>MSTLKNTFFITPPDTPTQAGPENIFYDFNDGARVLLPEGKWHVRLLDADSENILFCCDVDKGWVTSSKKYFVRFRIQVFRQGAATPLLDETLKLKDRPVLISFPTGTLGDLLGWFPYAERFQSLHKCRLECTMSQDIIDLLAPQYPQIQFSTPDKPRTVAPYATYRVGLYFGGDTNNQPVDFRKVGFHRSAGYILGVDPREAPVRLDLSAPRVIAAPYVCIATQSTCQAKYWNNGTGWSEVIAHLKSLGYRVMCIDRDAHYGQGFVWNHIPWGAEDFTGKLPLQERVNLLRHA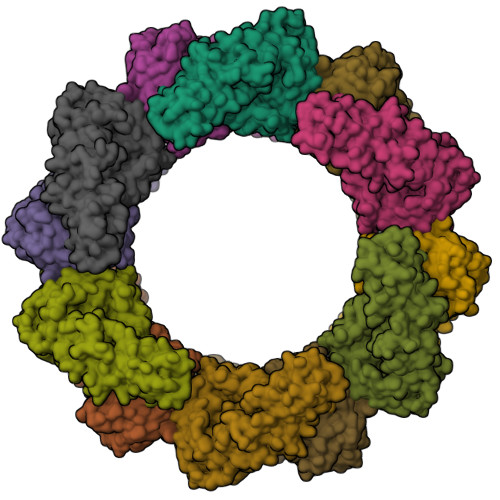SFFIGLPSGLSWLAWATRIPVVLISGFSLPNSEFYTPWRVFNSHGCYGCWDDTSLNFDHHDFLWCPRHKNTDRQFECTRLITGAQVNGVINKLHRSLTEQGVEATLAAGVSNE[12x]> TTIVALKYPGGVVMAGDRRSTQGNMISGRDVRKVYITDDYTATGIAGTAAVAVEFARLYAVELEHYEKLEGVPLTFAGKINRLAIMVRGNLAAAMQGLLALPLLAGYDIHASDPQSAGRIVSFDAAGGWNIEEEGYQAVGSGSLFAKSSMKKLYSQVTDGDSGLRVAVEALYDAAD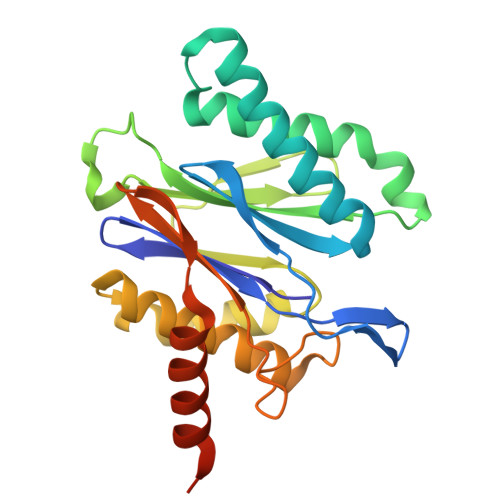DDSATGGPDLVRGIFPTAVIIDADGAVDVPESRIAELARAIIESRSGADTFGSDGGEK6-(1-methylbenzimidazol-4-yl)-3-[(4-morpholin-4-ylphenyl)amino]pyrazine-2-carboxamide 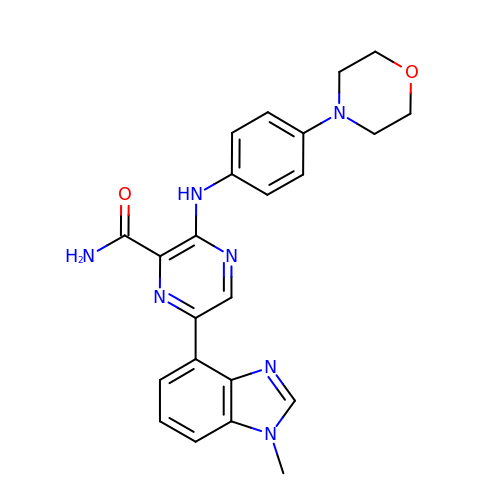| C23 H23 N7 O2 | AFUGKASDRSHPJZ-UHFFFAOYSA-N>[4x]GSSHHHHHHSSGRENLYFQGHMEFRPEMLQGKKVIVTGASKGIGREMAYHLAKMGAHVVVTARSKETLQKVVSHCLELGAASAHYIAGTMEDMTFAEQFVAQAGKLMGGLDMLILNHITNTSLNLFHDDIHHVRKSMEVNFLSYVVLTVAALPMLKQSNGSIVVVSSLAGKVAYPMVAAYS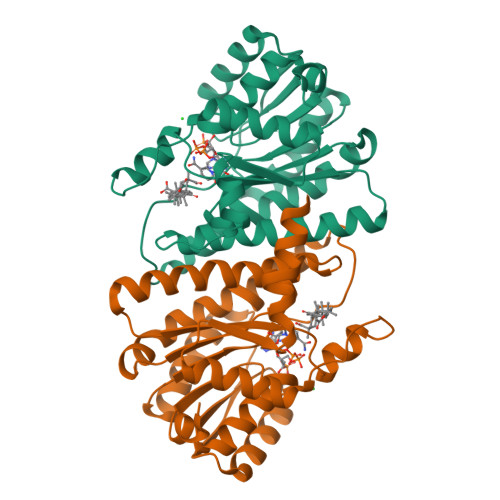ASKFALDGFFSSIRKEYSVSRVNVSITLCVLGLIDTETAMKAVSGIVHMQAAPKEECALEIIKGGALRQEEVYYDSSLWTTLLIRNPCRKILEFLYSTSYGS> PISPIETVPVKLKPGMDGPKVKQWPLTEEKIKALVEICTEMEKEGKISKIGPENPYNTPVFAIKKKDSTKWRKLVDFRELNKRTQDFWEVQLGIPHPAGLKKKKSVTVLDVGDAYFSVPLDEDFRKYTAFTIPSINNETPGIRYQYNVLPQGWKGSPAIFQSSMTKILEPFKKQNPDIVIYQYMDDLYVGSDLEIGQHRTKIEELRQHLLRWGLTTPDKKHQKEPPFLWMGYELHPDKWTVQPIVLPEKDSWTVNDIQKLVGKLNWASQIYPGIKVRQLSKLLRGTKALTEVIPLTEEAELELAENREILKEPVHGVYYDPSKDLIAEIQKQGQGQWTYQIYQEPFKNLKTGKYARMRGAHTNDVKQLTEAVQKITTESIVIWGKTPKFKLPIQKETWETWWTEYWQATWIPEWEFVNTPPLVKLWYQLEKEPIVGAETFYVDGAANRETKLGKAGYVTNKGRQKVVPLTNTTNQKTELQAIYLALQDSGLEVNIVTDSQYALGIIQAQPDKSESELVNQIIEQLIKKEKVYLAWVPAHKGIGGNEQVDKLVSAGIRKIL;> PISPIETVPVKLKPGMDGPKVKQWPLTEEKIKALVEICTEMEKEGKISKIGPENPYNTPVFAIKKKDSTKWRKLVDFRELNKRTQDFWEVQLGIPHPAGLKKKKSVTVLDVGDAYFSVPLDEDFRKYTAFTIPSINNETPGIRYQYNVLPQGWKGSPAIFQSSMTKILEP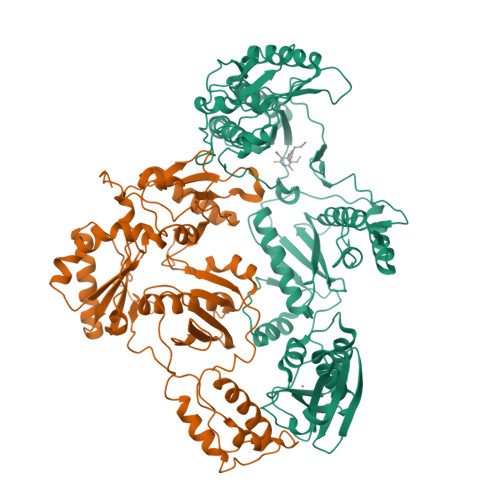FKKQNPDIVIYQYMDDLYVGSDLEIGQHRTKIEELRQHLLRWGLTTPDKKHQKEPPFLWMGYELHPDKWTVQPIVLPEKDSWTVNDIQKLVGKLNWASQIYPGIKVRQLSKLLRGTKALTEVIPLTEEAELELAENREILKEPVHGVYYDPSKDLIAEIQKQGQGQWTYQIYQEPFKNLKTGKYARMRGAHTNDVKQLTEAVQKITTESIVIWGKTPKFKLPIQKETWETWWTEYWQATWIPEWEFVNTPPLVKLWYQLE> GGPEAAAFVKVSMDGAPYLRKIDLRMYKSYDELSNALSNMFSSFTMGKHGGEEGMIDFMNERKLMDLVNSWDYVPSYENKDGNWMLVGDVPWPMFVDT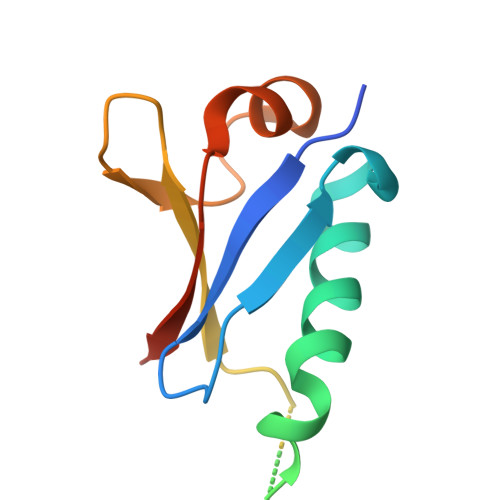AKRLRLMKGSDAIGL7-[2-(4-chlorophenoxy)ethyl]guanosine 5'-(dihydrogen phosphate) | C18 H22 Cl N5 O9 P | 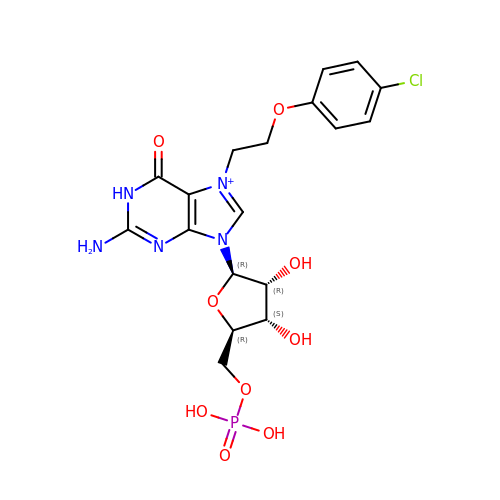QWFXGVANFMDSMH-LSCFUAHRSA-O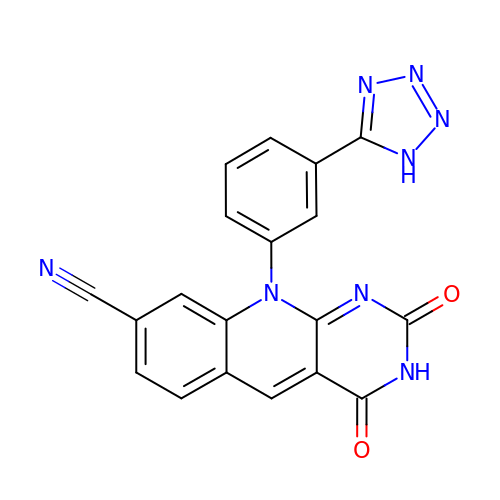2,4-dioxo-10-[3-(1H-tetrazol-5-yl)phenyl]-2,3,4,10-tetrahydropyrimido[4,5-b]quinoline-8-carbonitrile | C19 H10 N8 O2 | NDVGJTJBERLSGL-UHFFFAOYSA-N1-PHENYLSULFONAMIDE-3-TRIFLUOROMETHYL-5-PARABROMOPHENYLPYRAZOLE | C16 H11 Br F3 N3 O2 S | 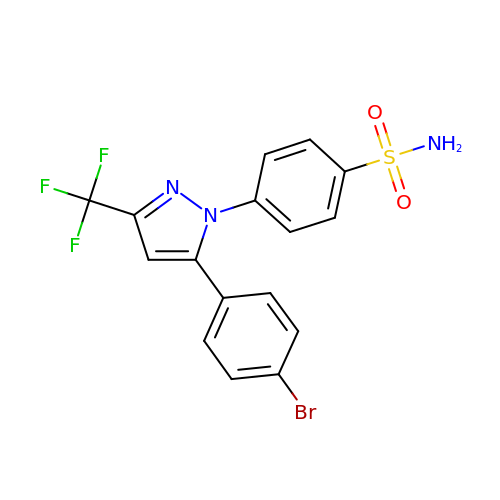OYZKFVIVPRQRQQ-UHFFFAOYSA-N>[4x]GAMEVAVLAESELGSEAQRERRKRILDATMAIASKGGYEAVQMRAVADRADVAVGTLYRYFPSKVHLLVSALGREFSRIDAKTDRSAVAGATPFQRLNFMVGKLNRAMQR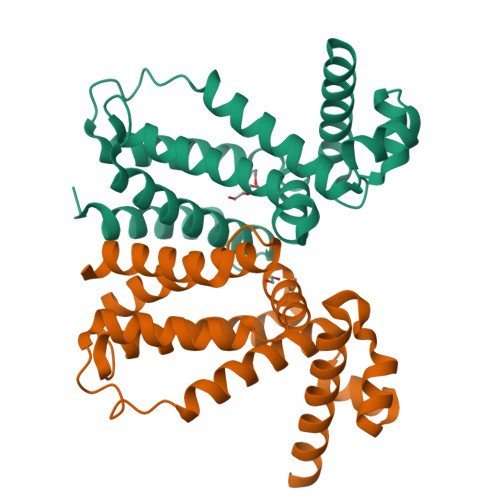NPLLTEAMTRAYVFADASAASEVDQVEKLIDSMFARAMANGEPTEDQYHIARVISDVWLSNLLAWLTRRASATDVSKRLDLAVRLLIGDQDSA> MGS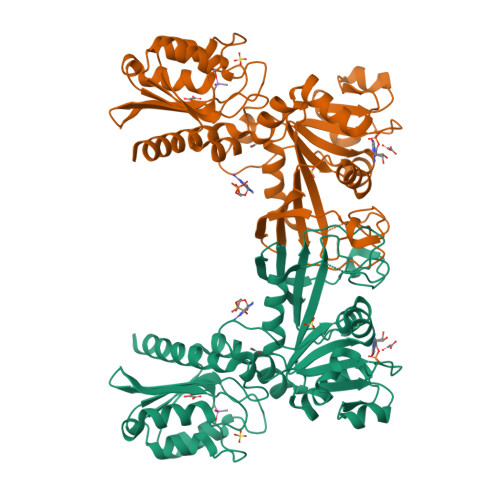SHHHHHHSSGENLYFQGHMSELKQDQYWMQQAIELAKRGLYSTKPNPNVGCVIVKDDQLIGEGFHPKAGQPHAEVFALRQAGEQAQGATAYVTLEPCAHYGRTPPCAEALVKAQVKKVVVACPDPNPLVAGKGVQILKNAGIEVEIGICEDLAAKLNQGFLKAMSTGMPYVRLKVASSLDGRTAMASGESKWITGSAARQDVQHWRAISGAVITGIDTVIADDCQLNVRSLHNIDIETVAQPKRVILDRRGRLPLTAKILENPETVMVMGPYRQELADLGVIQLEIQPLKTLLQTLSKQYQIYDVLIEAGATLSSAFLQEGLIDEMISYVAPTLLGQSARAMFNADFEYMAQQLRFKLLDVIQLDQDIRLRLIPTQEKV>[4x]DHYNCV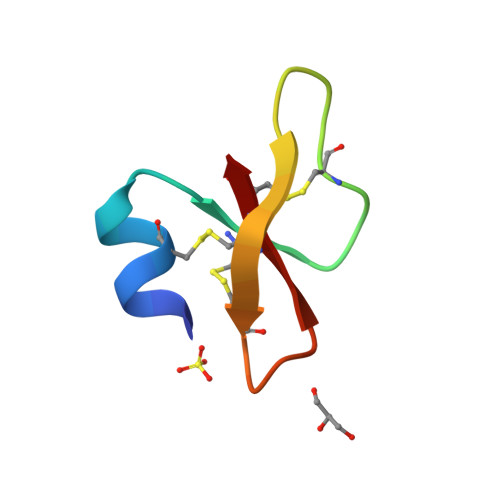SSGGQCLYSACPIFTKIQGTCYRGKAKCCK Oxypurinol | C5 H4 N4 O2 | 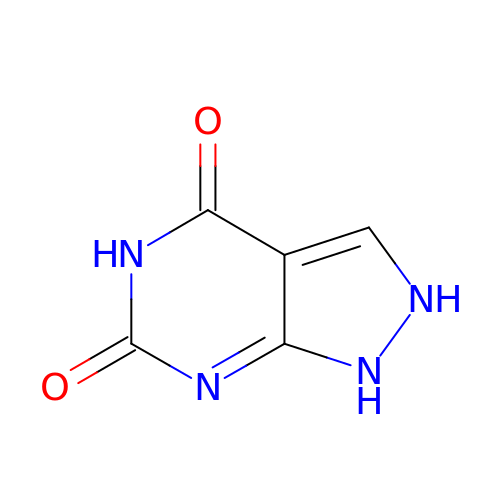HXNFUBHNUDHIGC-UHFFFAOYSA-N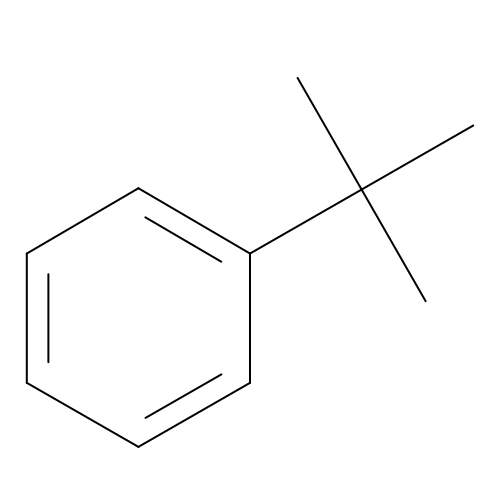tert-butylbenzene | C10 H14 | YTZKOQUCBOVLHL-UHFFFAOYSA-N Botulinum neurotoxins (BoNT) are a group of clostridial toxins that cause the potentially fatal neuroparalytic disease botulism. BoNTs are composed of three domains—a cell-binding domain, a translocation domain, and a catalytic domain. For BoNT/A, the HC/A binds to both a ganglioside (e.g., GD1a) and synaptic vesicle protein 2 (SV2C) at the nerve terminals of the neuromuscular junction. In this paper, we present the crystal structures of the botulinum neurotoxin A2 cell binding domain, both alone and in complex with its receptor ganglioside GD1a at 1.63 and 2.10 Å, respectively.

The structure of HC/A2 was determined to a resolution of 1.63 Å by molecular replacement. It has an N-terminal β-jelly roll fold and a C-terminal β-trefoil that is consistent with other HC/A subtypes. The quality of the electron density map is good throughout except for a small loop region (Arg 1269-Phe 1277). This loop (which is conserved across all BoNT/A subtypes) precedes the ganglioside binding site (GBS) and appears to be disordered for other HC/A subtypes. In both the HC/A2 and HC/A2:GD1a structures, clear electron density was observed between Lys 1236 and Cys 1280 indicating the presence of an unusual covalent bridge between the two residues. However, it was not possible to determine the identity of the bridging atom; crystallographically, both were equally possible. Further, a recent report based on a systematic study on the presence of Lys-Cys bridges in protein structures revealed that oxygen is the most likely bridging atom; therefore, we modelled this atom in the final deposited coordinates. Although the biological relevance of this Lys 1236-O-Cys 1280 bridge in the present HC/A2 structure is currently unknown, it is interesting to note that both these equivalent residues are conserved in all subtypes of BoNT/A, and that they are situated in a dynamic region of the protein close to the GBS.

> MHHHHHHKNIVNTSILSIVYKKDDLIDLSRYGAKINIGDRVYYDSIDKNQIKLINLESSTIEVILKNAIVYNSMYENFSTSFWIKIPKYFSKINLNNEYTIINCIENNSGWKVSLNYGEIIWTLQDNKQNIQRVVFKYSQMVNISDYINRWIFVTITNNRLTKSKIYINGRLIDQKPISNLGNIHASNKIMFKLDGCRDPRRYIMIKYFNLFDKELNEKEIKDLYDSQSNSGILKDFWGNYLQYDKPYYMLNLFDPNKYVDVNNIGIRGYMYLKGPRGSVVTTNIYLNSTLYEGTKFIIKKYASGNEDNIVRNNDRVYINVVVKNKEYRLATNASQAGVEKILSALEIPDVGNLSQVVVMKSKDDQGIRNKCKMNLQDNNGNDIGFIGFHLYDNIAKLVASNWYNRQVGKASRTFGCSWEFIPVDDGWGESSL> DNDSAPKEPTGPVTLIFTDIESSTALWAAHPDLMPDAVATHHRLIRSLITRYECYEVKTVGDSFMIASKSPFAAVQLAQELQLCFLRLDWETNAVDESYREFEEQRAEGECEYTPPTASLDPEVYSRLWNGLRVRVGIHTGLCDIRYDEVTKGYDYYGRTSNMAARTESVANGGQVLMTHAAYMSLSGEDRN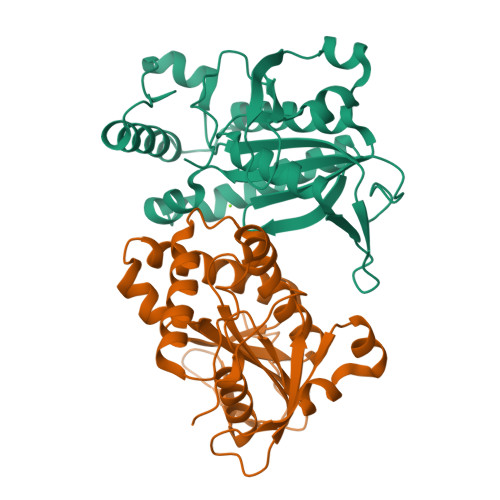QLDVTTLGATVLRGVPEPVRMYQLNAVPGRNFAALRLDR> PQ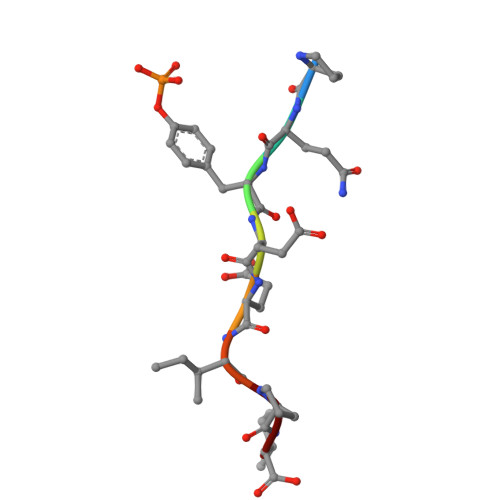YEEIPI During cell growth, PG endopeptidases cleave the crosslinks of the fully closed sacculi, allowing for the incorporation of new glycan strands and expansion of the peptidoglycan mesh. Outer-membrane-anchored NlpI associates with hydrolases and synthases near PG synthesis complexes, facilitating spatially close PG hydrolysis. The protein level of MepS is known to be regulated by the periplasmic PDZ-protease Prc (or tsp, tail-specific protease) in complex with the adaptor NlpI42. The structure of NlpI in complex with MepS provides molecular insight into NlpI-interacting endopeptidase colocalization, while the Prc-NlpI-MepS complex elucidates the molecular mechanism of NlpI-mediated MepS degradation by the tail-specific protease Prc.

To understand how NlpI enhances the efficiency of mMepS proteolysis by Prc, we determined the crystal structure of PrcSK-mMepS-NlpI at 3.5 Å, revealing that two monomeric PrcSK binds to heterohexameric NlpI-mMepS to form a 2:2:4 heterooctameric complex. We also examined the stoichiometry of the PrcSK-mMepS-NlpI complex through simultaneous SAXS and UV–Vis absorption measurements. The results showed that two monomeric PrcSK molecules bind to heterohexameric NlpI-mMepS, forming a 2:2:4 hetero-octameric complex measured at the eluent peak, with a confidence level exceeding 90%. Although the side-chain orientations can be easily defined in both NlpI and mMepS, the density maps of Prc are quite poor, except for the residues 42–120 (the N-terminal of NHD), 208–244 (the vault region) and 479–520 (the partial platform domain). The NlpI-interaction domain comprising helix h1 (residues 42–56) and helix h14 (residues 488–494) of Prc involved in interacting with NlpI can be well defined and almost identical between the structures of PrcSK-NlpI-MepS and NlpI-Prc-K477A. Unfortunately, the ligand-binding PDZ domain of PrcSK is poorly defined in the density map of the PrcSK-NlpI-MepS complex, suggesting that the ligand-binding PDZ domain is highly dynamic. The helix h9 of Prc can be clearly observed in our PrcSK-NlpI-mMepS and can be well superimposed with that of Prc-K477A in complex with NlpI, confirming that PrcSK adopts the active conformation in the PrcSK-NlpI-MepS complex. Moreover, in each PrcSK, we observed a co-purified peptide at the proteolytic site, with the unidentified peptide represented by a poly-Ala model. Owing to the missing electron density of  the ligand-binding PDZ domain, neither the position of PDZ domain nor the distance between the C-terminus of mMepS and the PDZ domain can be clearly determined. Overall, this study advances our knowledge of how NlpI recruits multiple MepS molecules and reveals the essential structural details required to understand the mechanism of NlpI-enabled MepS colocalization.

>[2x]MGSSHHHHHHSSGENLYFQGHMSNTSWRKSEVLAVPLQPTLQQEVILARMEQILASRALTDDERAQLLYERGVLYDSLGLRALARNDFSQALAIRPDMPEVFNYLGIYLTQAGNFDAAYEAFDSVLELDPTYNYAHLNRGIALYYGGRDKLAQDDLLAFYQDDPNDPFRSLWLYLAEQKLDEKQAKEVLKQHFEKSDKEQWGWNIVEFYLGNISEQTLMERLKADATDNTSLAEHLSETNFYLGKYYLSLGDLDSATALFKLAVANNVHNFVEHRYALLELSLLGQDQDDLAESDQQ;>[2x]MNMFFRLTALAGLLAIAGQTFAVEDITRADQIPVLKEETQHATVSERVTSRFTRSHYRQFDLDQAFSAKIFDRYLNLLDYSHNVLLASDVEQFAKKKTELGDELRSGKLDVFYDLYNLAQKRRFERYQYALSVLEKPMDFTGNDTYNLDRSKAPWPKNEAELNALWDSKVKFDELSLKLTGKTDKEIRETLTRRYKFAIRRLAQTNSEDVFSLAMTAFAREIDPHTNYLSPRNTEQFNTEMSLSLEGIGAVLQMDDDYTVINSMVAGGPAAKSKAISVGDKIVGVGQTGKPMVDVIGWRLDDVVALIKGPKGSKVRLEILPAGKGTKTRTVTLTRERIRLEDRAVKMSVKTVGKEKVGVLDIPGFYVGLTDDVKVQLQKLEKQNVSSVIIDLRSNGGGALTEAVSLSGLFIPAGPIVQVRDNNGKVREDSDTDGQVFYKGPLVVLVDRFSAAASEIFAAAMQDYGRALVVGEPTFGAGTVQQYRSLNRIYDQMLRPEWPALGSVQYTIQKFYRVNGGSTQRKGVTPDIIMPTGNEETETGEKFEDNALPWDSIDAATYVKSGDLTAFEPELLKEHNARIAKDPEFQNIMKDIARFNAMKDKRNIVSLNYAVREKENNEDDATRLARLNERFKREGKPELKKLDDLPKDYQEPDPYLDETVNIALDLAKLEKARPAEQPAPVKHHHHHH;>MSANNTAKNMHPETRAVGSETSSLQASQDEFENLVRNVDVKSRIMDQYADWKGVRYRLGGSTKKGIDCSGFVQRTFREQFGLELPRSTYEQQEMGKSVSRSNLRTGDLVLFRAGSTGRHVGIYIGNNQFVHASTSSGVIISSMNEPYWKKRYNEARRVLSRSHHHHHH[4x]>[4x]MSLTITPLSPALGAQISGVDISRDI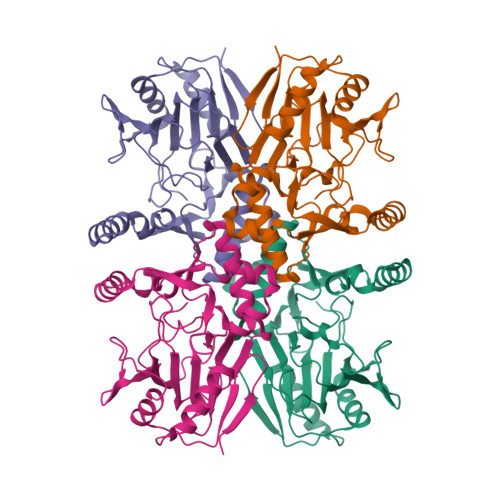SAEERDAIEQALLQHQVLFLRDQPINPEQQARFAARFGDLHIHPIYPNVPDTPQVLVLDTAVTDVRDNAVWHTDVTFLPTPALGAVLSAKQLPAYGGDTLWASGIAAFEALSAPLREMLDGLTATHDFTKSFPLERFGTTPQDLARWEATRRNNPPLSHPVVRTHPVSGRKALFVNEGFTTRINELSELESDALLRLLFAHATRPEFSIRWRWQENDVAFWDNRVTQHFAVDDYRPNRRVMHRATILGDAPF(1r,2r,3r,4r,5r,6r)-cyclohexane-1,2,3,4,5,6-hexol | C6 H12 O6 | 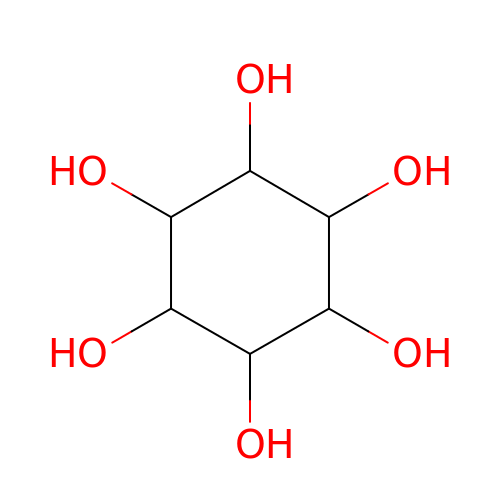CDAISMWEOUEBRE-CDRYSYESSA-N Phototransduction in retinal rods occurs when the G protein–coupled photoreceptor rhodopsin triggers the activation of phosphodiesterase 6 (PDE6) by GTP-bound alpha subunits of the G protein transducin (GαT). PDE6 consists of two highly similar but not identical subunits (PDE6α and PDE6β, Mr ∼100 kDa), each containing a catalytic site and two domains (GAFa and GAFb) that mediate a negative allosteric regulation by cGMP, together with two smaller (identical) subunits (PDE6γ, Mr ∼10 kDa) that are the binding sites for GTP-bound GαT (GαT·GTP). PDE6 is a 3′,5′-cyclic nucleotide phosphodiesterase and a member of a superfamily of enzymes that play critical roles in compartmentalizing cyclic nucleotide signaling and regulating many physiological processes. PDE6 is the most catalytically active PDE and is the only family member that has coevolved an autoinhibitory PDE6γ subunit, which enables G-protein–stimulated activation and completely prevents basal activity in the absence of GαT.

To see how this inhibitor affects the structural features of PDE6, we first determined a high-resolution reconstruction of the cryo-EM structure for the PDE6 holoenzyme alone. The resulting 3.1 Å cryo-EM map shows that the overall structure of the PDE6 heterotetramer is in good agreement with the cryo-EM structure of the PDE6 holoenzyme determined by Gulati et al. By combining the improved cryo-EM map with ModelAngelo, a newly developed graph neural network-based approach for automated model building, we were able to assign residues to a previously unbuilt region of the PDE6γ subunit and present a more complete structural model of the PDE6 holoenzyme. Strong cryo-EM density for residues Pro55 to Met57 allowed for the identification of a new hydrogen bonding network between the glycine-rich region of PDE6γ (residues 55–62) and the dimerization interface of the adjacent PDE6 catalytic subunit. PDE6γ residues Phe50, Asp52, Pro55, and Thr62 form hydrogen bonds with PDEβ residues Glu249, Arg255, His258, and Asp252, respectively, through interactions both between side chains and with the polypeptide backbone. Notably, despite its intrinsically disordered nature, PDE6γ adopts a largely stable conformation and remains tightly associated with the PDE6αβ subunit core across all variability components. For the PDE6 heterotetramer, the first variability component resolves bending of the PDE6α GAF domains toward the PDE6β catalytic core, which is associated with destabilization of the “ponytail motif”. Our high-resolution structure of PDE6 holoenzyme revealed a detailed interaction network between the glycine-rich region of PDE6γ and the PDE6α/β dimerization interface. Our high-resolution structure reveals that PDEβ H258 makes a critical hydrogen bond with the peptide backbone of PDE6γ P55.

> MGEVTAEEVEKFLDSNVSFAKQYYNLRYRAKVISDLLGPREAAVDFSNYHALNSVEESEIIFDLLRDFQDNLQAEKCVFNVMKKLCFLLQADRMSLFMYRARNGIAELATRLFNVHKDAVLEECLVAPDSEIVFPLDMGVVGHVALSKKIVNVPNTEEDEHFCDFVDTLTEYQTKNILASPIMNGKDVVAIIMVVNKVDGPHFTENDEEILLKYLNFANLIMKVFHLSYLHNCETRRGQILLWSGSKVFEELTDIERQFHKALYTVRAFLNCDRYSVGLLDMTKQKEFFDVWPVLMGEAPPYAGPRTPDGREINFYKVIDYILHGKEDIKVIPNPPPDHWALVSGLPTYVAQNGLICNIMNAPSEDFFAFQKEPLDESGWMIKNVLSMPIVNKKEEIVGVATFYNRKDGKPFDEMDETLMESLTQFLGWSVLNPDTYELMNKLENRKDIFQDMVKYHVKCDNEEIQTILKTREVYGKEPWECEEEELAEILQGELPDADKYEINKFHFSDLPLTELELVKCGIQMYYELKVVDKFHIPQEALVRFMYSLSKGYRRITYHNWRHGFNVGQTMFSLLVTGKLKRYFTDLEALAMVTAAFCHDIDHRGTNNLYQMKSQNPLAKLHGSSILERHHLEFGKTLLRDESLNIFQNLNRRQHEHAIHMMDIAIIATDLALYFKKRTMFQKIVDQSKTYETQQEWTQYMMLDQTRKEIVMAMMMTACDLSAITKPWEVQSKVALLVAAEFWEQGDLERTVLQQNPIPMMDRNKADELPKLQVGFIDFVCTFVYKEFSRFHEEITPMLDGITNNRKEWKALADEYETKMKGLEEEKQKQQAANQAAAGSQHGGKQPGGGPASKSCCVQ;> MSLSEGQVHRFLDQNPGFADQYFGRKLSPEDVANACEDGCPEGCTSFRELCQVEESAALFELVQDMQENVNMERVVFKILRRLCSILHADRCSLFMYRQRNGVAELATRLFSVQPDSVLEDCLVPPDSEIVFPLDIGVVGHVAQTKKMVNVQDVMECPHFSSFADELTDYVTRNILATPIMNGKDVVAVIMAVNKLDGPCFTSEDEDVFLKYLNFGTLNLKIYHLSYLHNCETRRGQVLLWSANKVFEELTDIERQFHKAFYTVRAYLNCDRYSVGLLDMTKEKEFFDVWPVLMGEAQAYSGPRTPDGREILFYKVIDYILHGKEDIKVIPSPPADHWALASGLPTYVAESGFICNIMNAPADEMFNFQEGPLDDSGWIVKNVLSMPIVNKKEEIVGVATFYNRKDGKPFDEQDEVLMESLTQFLGWSVLNTDTYDKMNKLENRKDIAQDMVLYHVRCDREEIQLILPTRERLGKEPADCEEDELGKILKEVLPGPAKFDIYEFHFSDLECTELELVKCGIQMYYELGVVRKFQIPQEVLVRFLFSVSKGYRRITYHNWRHGFNVAQTMFTLLMTGKLKSYYTDLEAFAMVTAGLCHDIDHRGTNNLYQMKSQNPLAKLHGSSILERHHLEFGKFLLSEETLNIYQNLNRRQHEHVIHLMDIAIIATDLALYFKKRTMFQKIVDESKNYEDRKSWVEYLSLETTRKEIVMAMMMTACDLSAITKPWEVQSKVALLVAAEFWEQGDLERTVLDQQPIPMMDRNKAAELPKLQVGFIDFVCTFVYKEFSRFHEEILPMFDRLQNNRKEWKALADEYEAKVKALEEDQKKETTAKKVGTEICNGGPAPRSSTCRIL;>[2x]MNLEPPKAEIRSATRVMGGPVTPRKGPPKFKQRQTRQFKSKPPKKGVQGFGDDIPGMEGLGTDITVICPWEAFNHLELHELAQYGII>GAMKTFDFTGPLRPGKITPRRAVPSHILRPDYADRAGGVSASEEKDRGSKVKVYNIQFLHDDSKKTAEIQRIKTVCQLSREVLDIATAAAKPGITTDELDRIVHEATVERNMYPSPLNYYGFPKSVCTSVNEVICHGIPDSRELEEGDILNIDVSSYLNGFHGDLNETVFIGRPDDDSVRLVHAAYECLCAGIGVVKPEALYKQVGDAIEACASQYQCSVVRTYTGHGVGHLFHTSPTV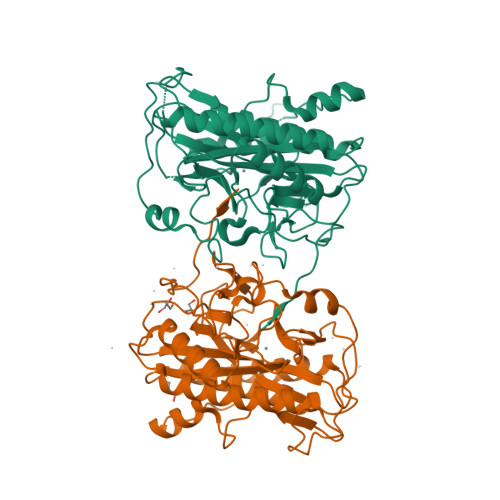CHYANNKSLGMMRPGHVFTIEPMINLGTWQDVTWPDKWTSTTKDGRRSAQFEHTMVVTNGGVEIFTDWVDGVPTYQKQLKEWGIMLPQRKEVGSATAV[2x]> MKLTLWTYEGPPHVGAMRVATAMKDLQLVLHGPQGATYADLLFTMIERRNARPPVSFSTFEASHMGTDTAILLKDALAAAHARYKPQAMAVALTCTAELLQDDPNGISRALNLPVPVVPLELPSYSRKENYGADETFRALVRALAVPMERTPEVTCNLLGATALGFRHRDDVAEVTKLLATMGIKVNVCAPLGASPDDLRKLGQAHFNVLMYPETGESAARHLERACKQPFTKIVPIGVGATRDFLAEVSKITGLPVVTDESTLRQPWWSASVDSTYLTGKRVFIFGDGTHVIAAARIAAKEVGFEVVGMGCYNREMARPLRTAAAEYGLEALITDDYLEVEKAIEAAAPELILGTQMERNIAKKLGLPCAVISAPVHVQDFPARYAPQMGFEGANVLFDTWVHPLVMGLEEHLLTMFREDFEFHDAAGASHHGGKAVAREESPVAPADLAPAATSDTPAAPSPVV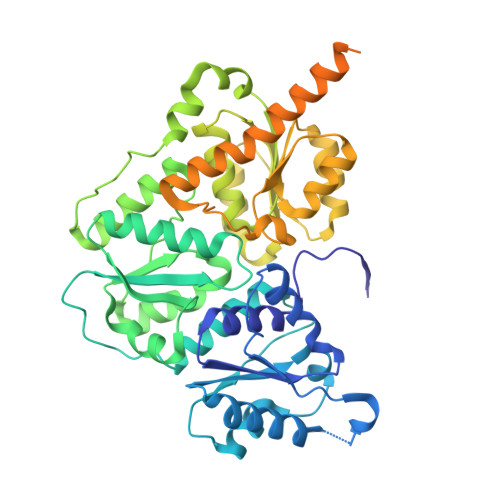VTQASGEIRWMPEAERELRKIPFFVRGKAKRNTELYAAHKGVCDITVETLYEAKAHYAR> ASKAAAPPPVRLFGVEGTYATALYQAAAKNSSIDAAFQSLQKVESTVKKNPKLGHLLLNPALSLKDRNSVIDAIVETHKNLDGYVVNLLKVLSENNRLGCFEKIASDFGVLNDAHNGLLKGTVTSAEPLDPKSFKRIEKALSASKLVGQGKSLKLENVVKPEIKGGLIVEL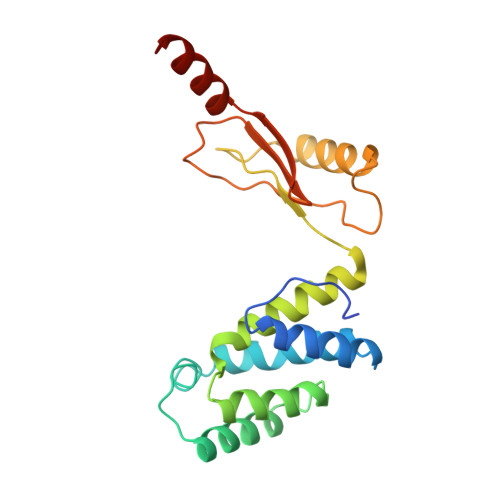GDKTVDLSISTKIQKLNKVLEDSI> QSSALRPSSLLRAYHYVHPKTGRPIRQYRKYGD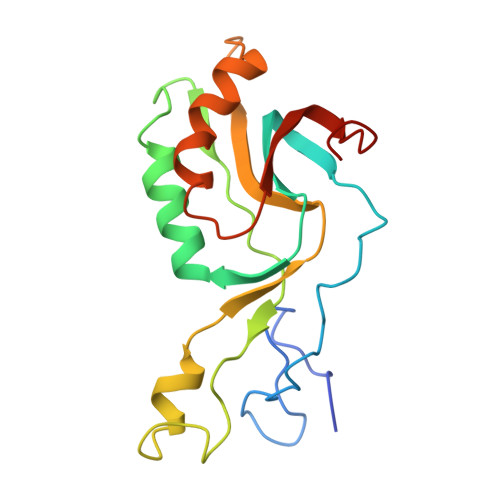PRFINNEVALIKGLFALITTDFGMVTQSQLENARLAILRRMPRGSFALTMHTDYEEFPVVQKSPESRMGAGKSNIHHFAYKFTTGVPLFEITALSSRRLNQAEAEGIFLAGRSFIPLQTAVVPRGRVDEYHVFK> QGMIICNNQIDDDQLKAIQDLASLCREHDGGTPTFYNHLLIQKRPTENNVLYFQDNQLLGFLSVYFFYEDACEVSLIVSPLHRRQGIAKQLLQTIMPLLTAKEMTTLIFSTPTEINDDWLINQGFSYRNSEYHMQRNGYDPIFMPTPKLHIRKATEDDIPALCAIDEACFPEHQENMISRFSMLLNDASYTLFLASYNHIIVGKAHIHWQSKEAIFSDIAIFPQYQGQGWGGELLSYCINQALTSGKNKLMLDVETSNQ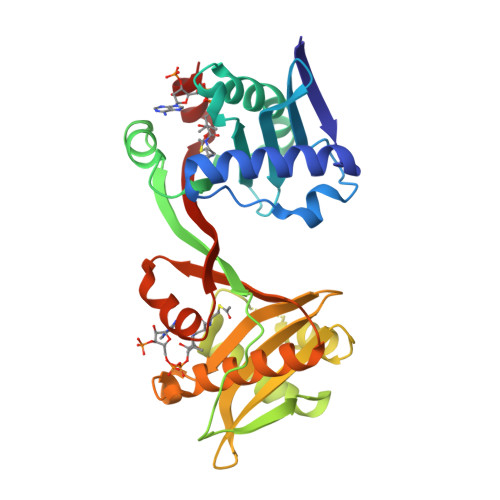NALHLYTRLGFKTANVSDYWVIPLPQLLTNWALE GCN5-related N-acetyltransferase (GNAT) toxin, with an acetyltransferase activity-dependent mechanism of translation inhibition, represents a relatively new and expanding family of type II TA toxins. We here describe a group of GNAT-Xre TA modules widely distributed among Pseudomonas species. Notably, other than arresting translation through acetylating aminoacyl-tRNAs, PacT can directly bind to Fur, a key ferric uptake regulator, to attenuate its DNA-binding affinity and thus permit the expression of downstream iron-acquisition-related genes. Previously studies on GNAT-RHH TA family also observed pronounced growth arrest after expression of the GNAT-type toxin and co-expression of its upstream antitoxin gene counteracted the toxic effect. It has been also demonstrated that the translational repression function of GNAT-type toxin depend on its acetyltransferase activity which transfers the acetyl group from acetyl coenzyme A (AcCoA) to the amine group of aa-tRNAs, subsequently resulting in the inhibition of translation.

In this study, we focused on a hypothetical P. aeruginosa TA pair pa3269/pa3270 that encodes a putative toxin PA3270 containing a GCN5-related N-acetyltransferase (GNAT) domain and a conserved acetyl-CoA-binding motif. This toxin has been hereafter referred to as PacT (Pseudomonas acetyltransferase toxin). The apo-form PacT exhibits a typical GNAT family fold consisting with a central, eight mixed β sheets which besieged by two or three α helices on each side. However, PacT exhibited low homology with GNAT-RHH toxins and the cognate antitoxin PacA bears a HTH (helix-turn-helix)-XRE (xenobiotic response element) motif; thus, PacTA was classified as a GNAT-Xre TA system. GNAT–RHH toxins, including E. coli AtaT and ItaT and S. Typhimurium TacT, have previously been reported to inhibit translation by acetylating charged tRNAs. These experimentally verified GNAT–RHH toxins only share 23.1%–25.53% identities with PacT, although all of them exhibit a conserved GNAT-fold and contain a unique motif (T/L-X-L/V/I-X5-G/K-X-G-L/F/W) for acetyl-coenzyme A binding. Taken together, these results confirmed that the PacT belongs to GNAT family and the PacTA constitutes a typical type II TA pair. According to the results, PacT directly bound to Fur. Next, we identified the interacting domain by using the truncated form Fur1-83 and found that this N-terminal DNA-binding domain could sufficiently mediate the Fur–PacT interaction. PacT can directly target the N-terminal HTH domain of Fur through protein–protein interactions without acetylation modification, but the binding of PacT obviously decreased the DNA-binding ability of Fur. Under iron starvation, the significantly increased PacT not only leads to overall translation inhibition and subsequent bacterial adaptation but also stimulates the iron uptake process by directly inhibiting the DNA-binding affinity of the negative iron acquisition regulator Fur.

>MSRRAPMFKPLPITLQRGALRLEPLVEADIPELVSLAEANREALQYMDGPTRPDWYRQSLAEQREGRALPLAVRLGVQLVGTTRFAEFLPALPACEIGWTWLDQAQHGSGLNRMIKYLMLKHAFDNLRMVRVQLSTAASNLRAQGAIDKLGAQREGVLRNHRRLAGGRLDDTFVYSITDHEWPQVKAALEASFTG[4x]>[2x]MAHHHHHHMRAYLDLLQHILDNGGDKGDRTGTGTRSVFGHQMRFDLSKGFPLLTTKKVHFRSIVIELLWFLKGDTNVKYLQDNKVTIWDEWATAEQTARFGRPEHELGPVYGHQWRNFGATKNADGTYNQDGFDQIKWLINE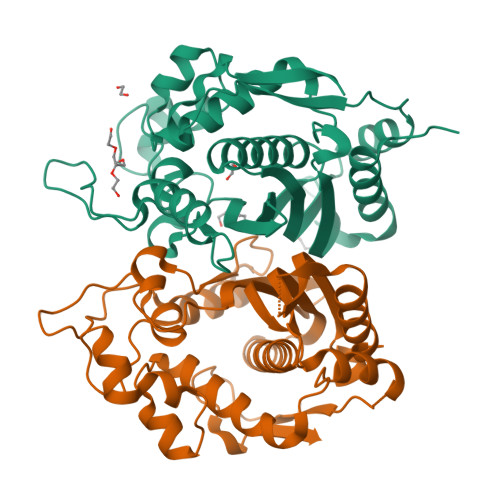IKTNPNSRRLIVSGWNPNEAGQVALPPCHTLFQFFVQDNKLSCQLYQRSADVFLGVPFNIASYALLTHMIAQVCGLGVGDFVWTGGDTHLYANHFEQAKLQLTREPLPLCQLKLNPEVKDIFDFKFEDIEIVGYESHPAIKAPVAV>GPKKISNCSKIHLSTKLLAVDFPAHFVKSISCQICEHILADPVETSCKHLFCRICILRCLKVMGSYCPSCRYPCFPTDLESPVKSFLNILNSLMVKCPAQDCNEEVSLEKYNHHVSSHKESKETLVHINKGGRPRQHLLSLTRRAQKHRLRELKIQVKEFADKEEGGDVKAVCLTLFLLALRARNEHRQADELEAIMQGRGSGLQPAVCLAIRVNTFLSCSQYHKMYRTVKAITGRQIFQPLHALRNAEKVLLPGYHPFEWQPPLKNVSSRTDVGIIDGLSGLASSVDEYPVDTIAKRFRYDSALVSALMDMEEDILEGMRSQDLDDYLNGPFTVVVKESCDGMGDVSEKHGSGPAVPEKAVRFSFTVMRITIEHGSQNVKVFEEPKPNSVLCCKPLCLMLADESDHETLTAILSPLIAEREAMKSSELTLEMGGIPRTFKFIFRGTGYDEKLVREVEGLEASGSVYICT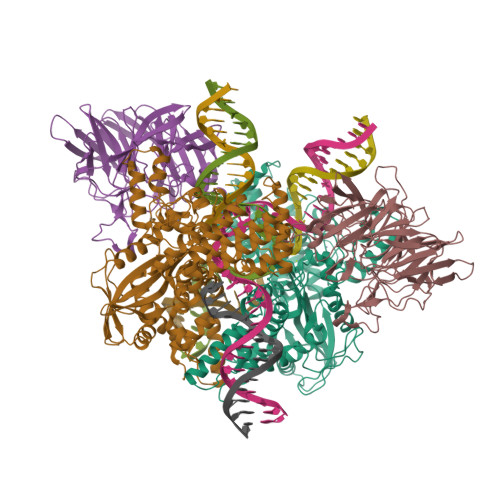LCDTTRLEASQNLVFHSITRSHAENLQRYEVWRSNPYHESVEELRDRVKGVSAKPFIETVPSIDALHCDIGNAAEFYKIFQLEIGEVYKHPNASKEERKRWQATLDKHLRKRMNLKPIMMMNGNFARKLMTQETVDAVCELIPSEERHEALRELMDLYLKMKPVWRSSCPAKECPESLCQYSFNSQRFAELLSTKFKYRYEGKITNYFHKTLAHVPEIIERDGSIGAWASEGNESGNKLFRRFRKMNARQSKCYEMEDVLKHHWLYTSKYLQKFMNAHNA[2x];>GPMALQMVTVGHNIALIQPGFSLMNFDGQVFFFGQKGWPKRSCPTGVFHFDIKQNHLKLKPAIFSKDSCYLPPLRYPATCSYKGSIDSDKHQYIIHGGKTPNNELSDKIYIMSVACKNNKKVTFRCTEKDLVGDVPEPRYGHSIDVVYSRGKSMGVLFGGRSYMPSTQRTTEKWNSVADCLPHVFLIDFEFGCATSYILPELQDGLSFHVSIARNDTVYILGGHSLASNIRPANLYRIRVDLPLGTPAVNCTVLPGGISVSSAILTQTNNDEFVIVGGYQLENQKRMVCSLVSLGDNTIEISEMETPDWTSDIKHSKIWFGSNMGNGTIFLGIPGDNKQAMSEAFYFYTLRCSEEDLSEDQKI[2x]> MGSSHHHHHHSQDPNSDFKLEQVLTSREWQSKMVSLIKTNSNRPAMGPLSRVDVTSNVKYLPNGTYLRVSIVKLFSDDNSAESVINISEFGEWDISDNYLLVTPVEFKDISSNQSKDFTDEQLQLITQLFKMDAQQSRRVDIVNERTILFTSLSHGSTV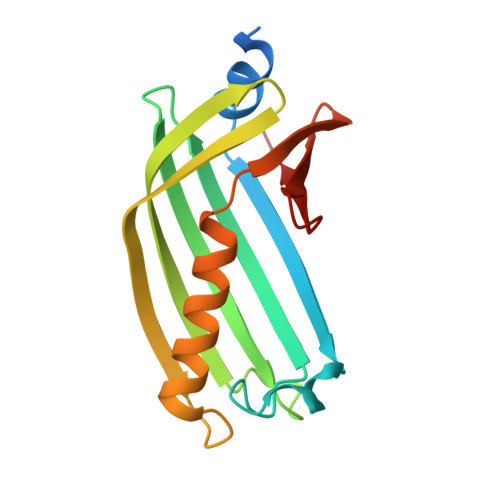LFSNS2,2-dimethylpropyl 2-[(3-oxidanylidene-5-sulfanylidene-2~{H}-1,2,4-triazin-6-yl)amino]ethanoate | C10 H16 N4 O3 S | 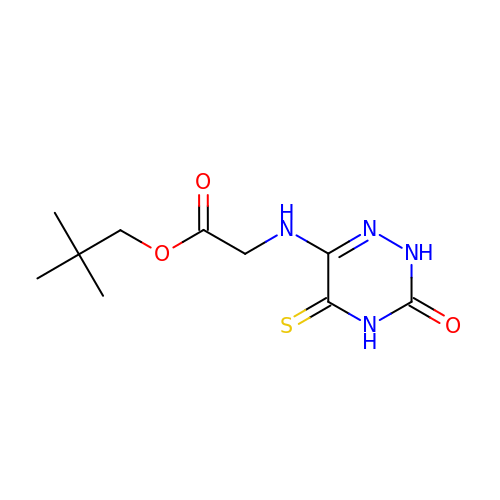REFYLRHEWINELP-UHFFFAOYSA-N> MTDKLIRELLIDVKQKGATRTAKSIENVSDALENAAAASELTNEQLGKMPKTLYSIERAADRAAKSLTKMQASRGMAGITKSIDSIGAKLDDLSIAMIEVADKLEAGFDGVSRSVKVMGNDVAAATEKVQDRLYDTNRVLGGTARGFNDTAGAAGRASRAIGNTSGSARGATRDFAAMAKVGGGLPLLYAAIASNIFVLQSAFEQLKLGDQLNRLEEFGVIVGTQTGTPVQSLARSLQEAAGYAISFEEAMRQASSASAYGFDAEQLNKFGLVARRAAAVLGVDMTDALNRVIKGVSKQEIELLDELGVTIRLNDAYADYVKQLNAANTGITYNINSLTTFQKQQAYANAVI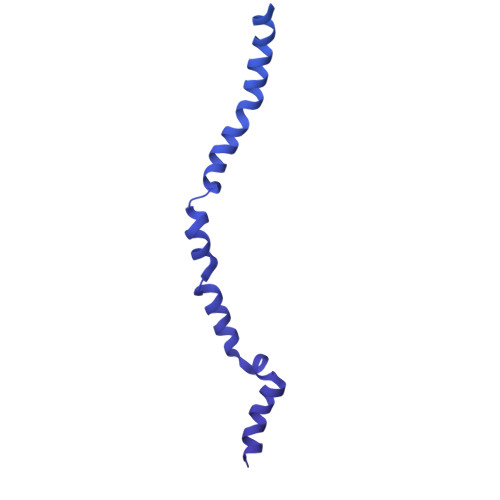AESTKRFGYLDEVLRATPWEQFAANADAALRTIQQAAAKYLGPVIDAINTVFYTSQASISAEAARAQEQTNKQIDPTNVGAVALSLSASEEGYNKALDMYKESLDKRNKLKSEFDKRMEQADFYTKLAIRQVGEGIPAGLATAGASEANKKFVEETAAMGLQVARLDKEVTDSTENLNAWKSAYQAAGAAAAKANPEFQKQINLQRDTTDPGAVYDFNSTVLKGLTEQQKAYNQTKKTASDLANDIQNVAQNTDTAAKTSATLADAIKNIESLSLGTGKSADEYVKNLNLGYNTLSEMKTASQALSEYVKLTGNETKNQLAVQQKIADVYNQTKDKEKAQEAGRRLELQQLEEQEAALRRVLQTNQGNKAVEREIEKIQLEKIKLTNQGMEAQKKVKDYTDKILGVDREIALLNNRTMTDTQYRLAQLNLELTIEKEKYEWYTKQADKQKEAEQSRRAQAQIEREIWKFHQDQQAEMTSKRQEAFENTLTSMFPLAGEMQKMEMQLDFYTQMKELTKDNANEQMRWNAEIAKTRAQMSALTAQRNAQMQSSVGSSLGAVYTPTTGLSGEDKKFADMGNQLASYDQAISKLSELNSEATAVAQSMGNLANAMIQFSQGSLDTTSTIAVGMQTVASMIQYSTSQQVSAIDQAIAAEQKRDGKSEASKAKLKKLEAEKLKIQQDAAKKQIIIQTAVAVMQAATAVPYPFSIPLMIAAGLAGALALAQASSASGMSSIGDSGADTASYLTLGERQKNIDVSMSANAGELSYVRGDKGIGNANSFVPRAEGGNMYPGVSYQMGEHGTEVVTPMVPMKATPNDELKNSSNSTAGRPIILNISAMDAASFREFASSNSGALRDAVELALNENGASLKTLGNS> MATKEQIV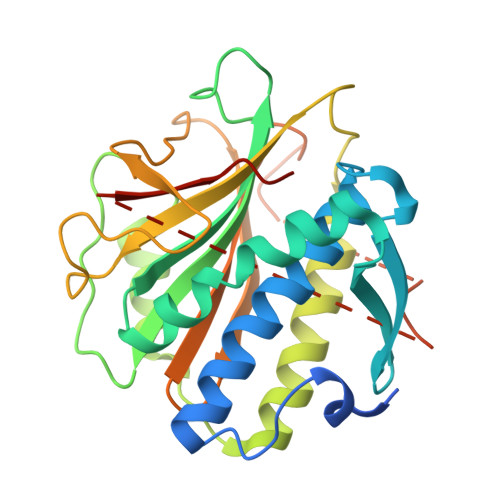EHRESEIPIASQWKATFPVDLEIEKNSEMFALRYIKCASAFILDRRGILDEKCFKTRTIDKLLVTAFQSSVPAAKRVSSTFDGLRDAIQQGYLREFAIVFYKKPNEEDINEVFAFRFAYGDEGEIFVSLNNGIDTNESSQELLQAKFVDTDNTKQMFASTIKKLHRCIKKMEPLPQGSDASFRVSYTEKAPKDYTPEGYLLSPMFYTLNQDIRKASIGIVCGGHHKIQMLAASQYLKQDFDLDKTTTLNPNMSIMANQSKRKGRISRDSPYGLSQGITKKNKD> NTLF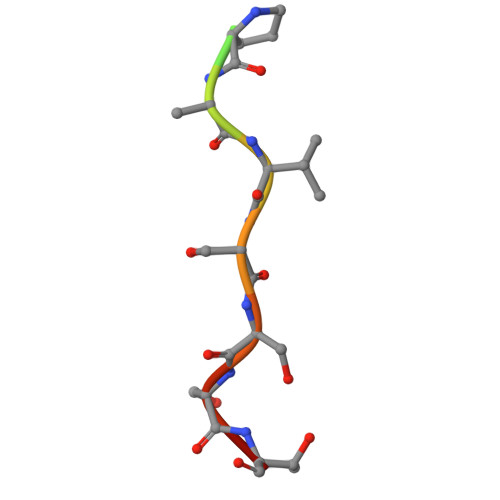PDVSSSTH> MLSRKGIIPEEYVLTRLAEDPAEPRYRTRERRARFVSKKGNCNVAHKNIREQGRFLQDVFTTLVDLKWPHTLLIFTMSFLCSWLLFAMVWWLIAFAHGDLAPGEGTNVPCVTSIHSFSSAFLFSIEVQVTIGFGGRMVTEECPLAILILIVQNIVGLMINAIMLGCIFMKTAQAKRRAETLIFSKHAVITLRHGRLCFMLRVGDLRKSMIISATIHMQVVRKTTSPEGEVVPLHQVDIPMENGVGGNGIFLVAPLIIYHVIDSNSPLYDLAPSDLHHHQDLEIIVILEGVVETTGITTQART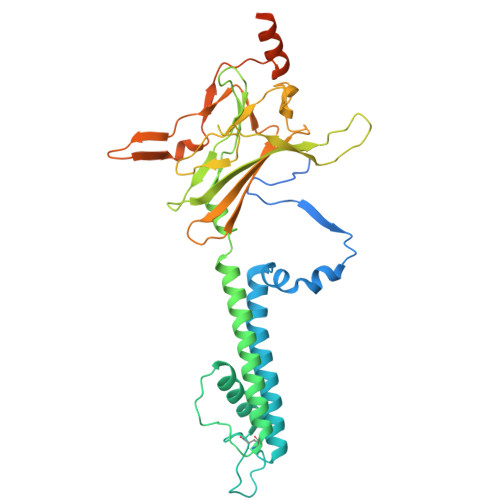SYLADEILWGQRFVPIVAEEDGRYSVDYSKFGNTIKVPTPLCTARQLDEDRSLLDALTLASSRGPLRKRSVAVAKAKPKFSISPDSLS> ETGVFQKAVDQSIEKKIVLRNGTEAFDSWEKPPLPVYTQFYFFNVTNPEEILRGETPRVEEVGPYTYRELRNKANIQFGDNGTTISAVSNKAYVFERDQSVGDPKIDLIRTLNIPVLTVIEWSQVHFLREIIEAMLKAYQQKLFVTHTVDELLWGYKDEILSLIHVFRPDISPYFGLFYEKNGTNDGDYVFLTGEDSYLNFTKIVEWNGKTSLDWWITDKCNMINGTDGDSFHPLITKDEVLYVFPSDFCRSVYITFSDYESVQGLPAFRYKVPAEILANTSDNAGFCIPEGNCLGSGVLNVSICKNGAPIIMSFPHFYQADERFVSAIEGMHPNQEDHETFVDINPLTGIILKAAKRFQINIYVKKLDDFVETGDIRTMVFPVMYLNESVHIDKETASRLKSMINTGTKHHHHHH

Lysosomal integral membrane protein 2 (LIMP-2) is encoded by gene SCARB2, and is also known as scavenger receptor class B member 2 (SCARB2; refs 1, 2). It has N- and C-terminal transmembrane helices (being a type III membrane protein) and a heavily glycosylated 400 residue luminal domain (bearing nine potential N-linked glycosylation sites). The most notable function of LIMP-2 is that it serves as a lysosomal sorting receptor for β-glucocerebrosidase (β-GCase), deficiency of which causes Gaucher disease, a lysosomal storage disease in which glucocerebrosides accumulate. LIMP-2 binds to β-GCase in a pH-dependent manner, and dissociation occurs in acidic late endosomal/lysosomal compartments.

Human LIMP-2 luminal domain containing residues 28–431 was produced by stable expression in HEK293S (GnTI−) cells and crystallized in two space groups, C2221 and C2, at pH 6.5. X-ray diffraction data were collected at the Diamond Light Source, and structures of both crystal forms were determined using the molecular replacement method based on the model of LIMP-2 at lower pH9 and refined at 2.8 Å resolution. The electron density maps for both space groups are of good quality with only 11 terminal residues disordered with 29 and 30 glycosidic units well ordered in the two space groups. The most surprising observation is that we can identify from the well-defined electron density that the sugar attached to N325 is P-Man9GlcNAc2, the first time this sugar, which bears a terminal M6P, has been seen in a protein structure. In the C2221 crystal, the sugars are also stabilized by interaction with residues from a symmetry-related molecule that pack directly at the origin of the three arms of the glycan, forming a network of hydrogen bonds, although this destabilizes the distal phosphate group. A well-defined ion (likely Na+) bridges the O2 atom of the β-mannose to O4 of the terminal D2 mannose (glycan nomenclature is defined in Supplementary Fig. 1a). Although our two structures at pH 6.5 are almost identical to each other (root mean squared deviation=0.3 Å for all Cα atoms), they differ significantly from the pH 5.5 structures (root mean squared deviation=0.5–0.6 Å), with the largest difference occurring in the helical bundle of domain II, which includes exactly the region (residues 150–167) identified as the β-GCase binding site. In contrast, at pH 6.5, the helical bundle is very well defined and similar in both space groups. At higher pH, the α4–α5 linker (residues 151–152) folds towards α7, such that α5 tilts about 20° towards α4 and α7, making the bundle more compact and further stabilized by the C-terminal cap of α4 formed by His150 and Arg153. At lower pH, H150 and R153 move away, decapping the α4 C terminus and triggering a cascade of structural change in the helical bundle that leads to the dissociation of β-GCase from LIMP-2.>[2x]MA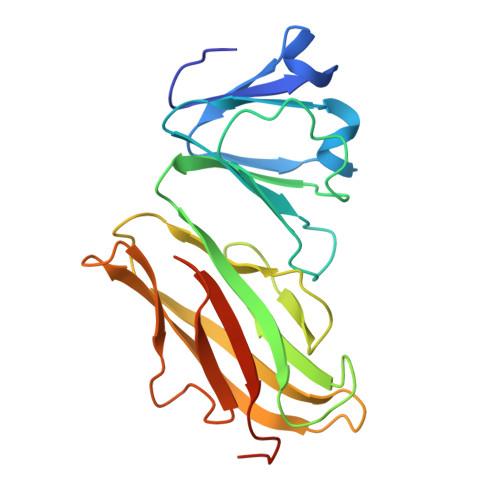PSVDPTKVIFYQKKNFEGSGDTYAVGQDVSVPGSLNDKYFSVAVGASAKVIAWQHYNETGHYREWTTSQADISDIGGLSRFRVVDDDTRAISFLFKDATGGADKQYSLKVDARDVGTVMLYSNDGDEYGLVGIMPEGGPPVTTAVYVRDEHSGVYIAVGSVYFEWNKDNGEVDVVENEHWPKQLKSKRTGKSSFEVTLVDNKPSELEHHHHHH naphthalene-2-carboxylic 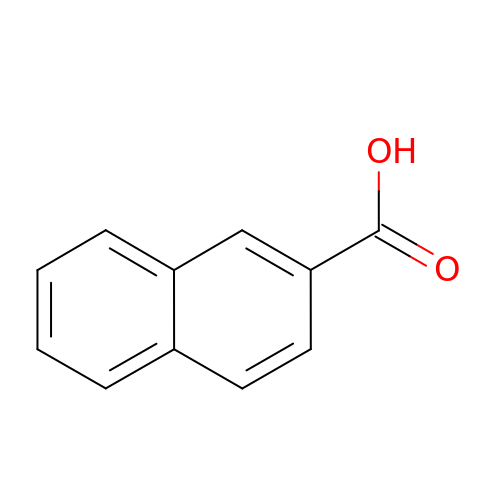acid | C11 H8 O2 | UOBYKYZJUGYBDK-UHFFFAOYSA-N>MHHHHHHHHHHMHHDKRCKESNMKIVKAEVFVTCPGRNFVTLKITTEDGITGLGDATLNGRELSVASYLQDHLCPQLIGRDAHRIEDIWQFFYKGAYWRRGPVTMSAISAVDMALWDIKAKAANMPLYQLLGGASREGVMVYCHTTGHSIDEALDDYARHQELGFKAIRVQCGIPGMKTTYGMSKGKGLAYEPATKGQWPEEQLWSTEKYLDFMPKLFDAVRNKFGFDEHLLHDMHHRLTPIEAARFGKSIEDYRMFWMEDPTPAENQECFRLIRQHTVTPIAVGEVFNSIWD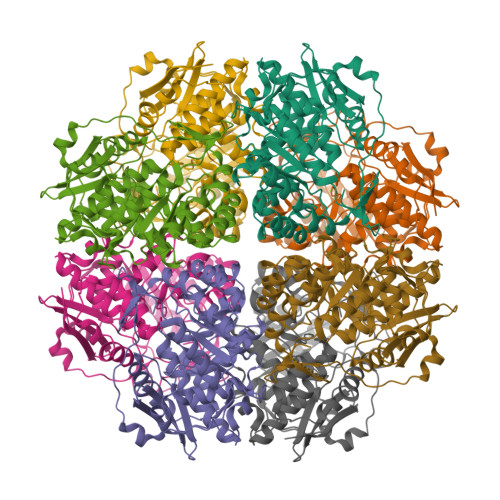CKQLIEEQLIDYIRTTLTHAGGITGMRRIADFASLYQVRTGSHGPSDLSPVCMAAALHFDLWVPNFGVQEYMGYSEQMLEVFPHNWTFDNGYMHPGEKPGLGIEFDEKLAAKYPYEPAYLPVARLEDGTLWNW[4x]> GTKFSKEQLRTFQMIHENFGRALSTYLSGRLRTFVDVEISIDQLTYEEFIRSVMIPSFIVIFTGDVFEGSAIFEMRLDLFYTMLDIIMGGPGENPPNRPPTEIETSIMRKEVTNMLTLLAQAWSDFQYFIPSIENVETNPQFVQIVPPNEIVLLVTASVSWGEFTSFINVCWPFSLLEPLLEKLSDR;> GHMDPVQLVNFLQSEHPQTIAVVLSYLD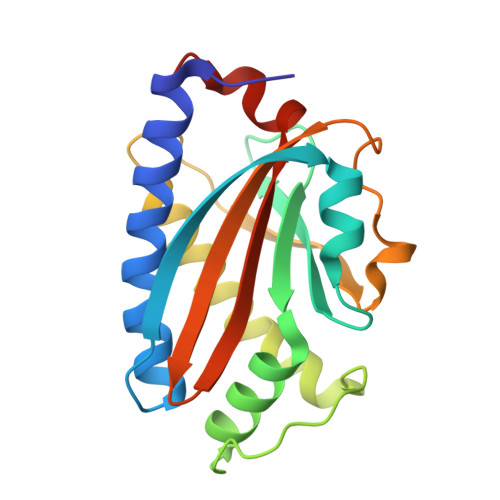PPVAAQILGALPEELQTEVLKRIALLERTSPEVVKEIERNLEKKISGFVSRTFSKVGGIDTAAEIMNNLDRTTEKKIMDKLVQENPELADEIRRRMFVFEDILKLDDRSIQLVLREVDTRDLALALKGASDELKEKIFKNMSKRAAALLKDELEYMGPVRLKDVEEAQQKIINIIRRLEEAGEIVIAR> MALPLDFTNSDVVMGALTKAVGRLCLDVTGYDVVEADETIPKPEGPYILVDLSLLTPLDWATNEVVDEDGVVHTAHNYTASYTLTAYRGKPHWALSRVHQAFGLPFLREKYFPTGSPYAYSSTSNIARMRVPLNQQMFENRARTIVTFNATFVEKDLGTFED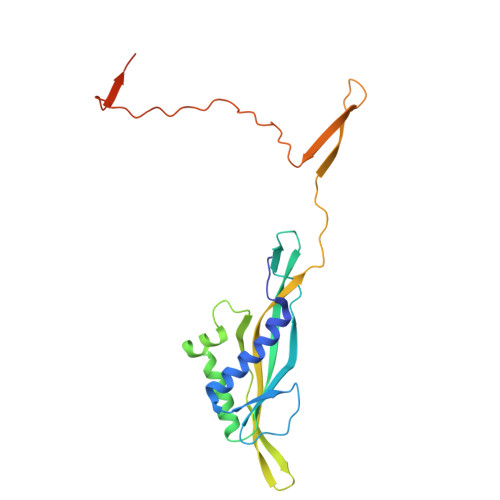IEHIIIGIDVDNPSGPPIGIGADYDKGVKPGGDDPGLPPKPNPPIVYHDAIAQVCMATPVIDKPALISDKTGE2-methyl-N-(pyridin-4-yl)furan-3-carboxamide | C11 H10 N2 O2 | 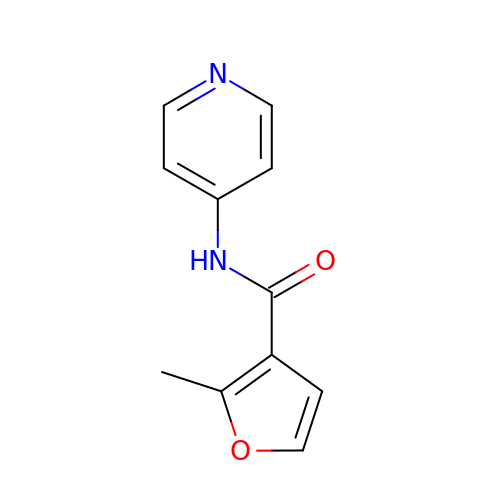YQBDLYFUZJNLDH-UHFFFAOYSA-N> ATFEIVNRCSYTVWAAASKGDAALDAGGRQLNSGESWTINVEP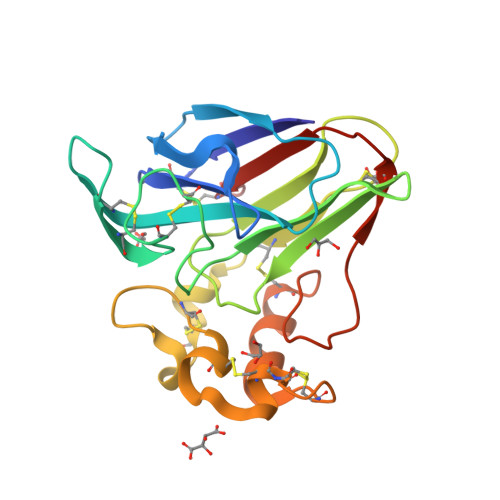GTNGGKIWARTDCYFDDSGSGICKTGDCGGLLRCKRFGRPPTTLAEFSLNQYGKDYIDISNIKGFNVPMDFSPTTRGCRGVRCAADIVGQCPAALKAPGGGCNDACTVFQTSEYCCTTGKCGPTEYSRFFKRLCPDAFSYVLDKPTTVTCPGSSNYRVTFCPTA> MSTKTKTIFDEIKAALVLKVIDSPLGRKLIEEKAEKQVSKTQEAITKPIEQLNKATGQLLFSDTNKPLHNIELEVWDRDVGTPSDYLGKGVTDQNGRFEIYYDPEKAGFKDAPDLELRVIDNRVTFDSDNQPVYTNRIAYIIKGGDNVTQKTYDFGTLTVPYWPYDPNSPFARIFMPNPEETPDDYSVGRKFQAYASANVLTPIKAKHTIANTLNPKEPSLTQIQADYPPNLTINLDREKPGYTRSDEYFVLRVLNGMNPCLLKRSKSDPNQFKMSFIWDNYEKDTEHDLHNVEAYFVLKDGKLFPTMITIQSRYPDSLAPHSPLKDREVYTPNDGEKWLQAKRIFRTAALFDGEAIEHYAKAHVQMEQY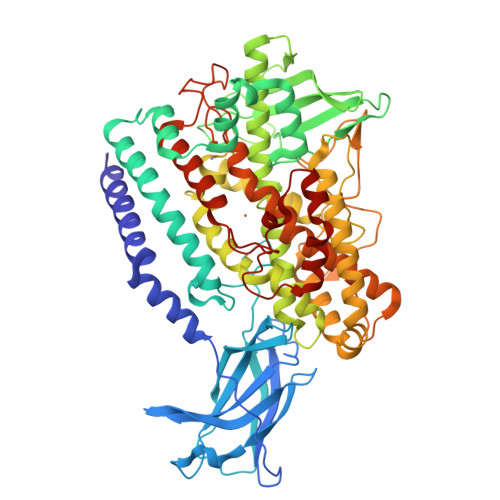AVACFRNLRKNPIRLMLTPHLKSIININRRGDDLLVEPNLGLFVTNGPLTYPGFLQMCTEVVATYDWKDWQPRQPICDDHKYAKAANLYWQILTEYVDAFFAKHQQAIADEWVEIRRFSEDLVEHSMPYQPIEGIMANTDSDYEWYDTGELDKPDLPRATFNGKTKVIRPITNSNQPSATDIDNLKQCCRHIIFHTTLWHTWVNDSQSDEGGELAYNSLALRNGSFGSETDPNIAPDPIEATNQVYIFSVLNGIKYGLLVKNEDDDVPEELRTALLNRKDQFAELGIDIGNIRTLINI N-acetyl sugar amidotransferase (NASAT) is involved in the lipopolysaccharide (LPS) biosynthesis pathway that catalyzes the formation of the acetamido moiety (sugar-NC(=NH)CH3) on the O-chain. The reaction involves the ligation of ammonia with a sugar N-acetyl group, displacing water. The NASAT family belongs to the AANH_like (Adenine nucleotide alpha hydrolases-like) superfamily, whose domain forms an alpha/beta/alpha fold for Adenosine nucleotide binding. Members of the NASAT family carry a conserved PP-loop (SGGXDS, where X represents any residue), indicating that they may have ATP PPase activity.

Here, we report the crystal structure of an N-acetyl sugar amidotransferase from Legionella pneumophila (LpNASAT) at 2.33 Å resolution. LpNASAT folds into a compact basin-shaped architecture with an unusually wide and open putative substrate-binding pocket and a conserved zinc ion-binding tetracysteine motif. A five-stranded parallel β-sheet (β3β2β1β4β7) in the core (lower part) of the molecule was sandwiched by two arrays of α-helices (α3α4α6α10α11), which is a typical nucleotide-binding Rossmann-like fold. On the edge of the pocket, there is a conserved tetracysteine motif (Cys44, Cys47, Cys79 and Cys82) possibly indicative of a metal binding site. To confirm the identity of the metal, we conducted inductively coupled plasma mass spectroscopy (ICP-MS) experiments on highly purified LpNASAT, and the results showed that zinc appears to be the candidate among the transition metals under investigation. Two LpNASAT molecules in the asymmetric unit seem to form a dimer. PISA (Proteins, Interfaces, Structures and Assemblies) program analysis of protein the interfaces suggests that the dimer is likely to be stable in solution with a favorable interaction energy (ΔiG −3.9 kcal/mol), consistent with the results of size exclusion chromatography. According to the electron density map, a fragment consisting of approximately fifteen residues (residues 55–69) is severely disordered. Therefore, we hypothesize that this region maybe be involved in the regulation of substrate binding and product release. At the bottom of the putative substrate-binding pocket, LpNASAT harbors a highly conserved PP-loop motif (122-SGGKDS-127) on a region between β1 and α3.

>[2x]MGHHHHHHMSNARIGIDMSKIYAPKSIDLSSFQLPDEKLQTKYGLPHKVEFCKSCVISNQRPNSAVEYEHKKESKKHTIHFDDEGICDACRVAERKKSTINWEERDRQLRELCDRFRSKDGSYDCVVPGSGGKDSFYAAHILKYKYGMNPLTVTWAPHMYTPWGWRNFQSWIHAGFDNHLFTPNGRVHRLLTRLAVENLFHPFQPFMIGQKAYAPKMALLHKIKLVVYGENEAEYGNPIGDTESAKRDWKYFTADDKSKIFLGGTSVQELKSDFGLNDNDLDAYLPADPQQIEEQQVEVHYLGYYLKWHPQSCYYYSVEHGGFEASPERTPGTYSKYNSIDDKIDDFHYYTTLTKFGIGRATYDASQEIRSGDITREEGVALVKRFDQEFPERFAEEIFKYLSINLKEFPIASQMFEQPIMDRAYFMALADTFRSPHLWKKDGEQWKLRHQVTNLEKTKAEYLDLETV>[2x]SMANLRKVLISDSLDPCCRKILQDGGLQVVEKQNLSKEELIAELQDCEGLIVRSATKVTADVINAAEKLQVVGRAGTGVDNVDLEAATRKGILVMNTPNGNSLSAAELTCGMIMCLARQIPQATASMKDGKWERKKFMGTELNGKTLGILGLGRIGREVATRMQSFGMKTIGYDPIISPEVSASFGVQQLPLEEIWP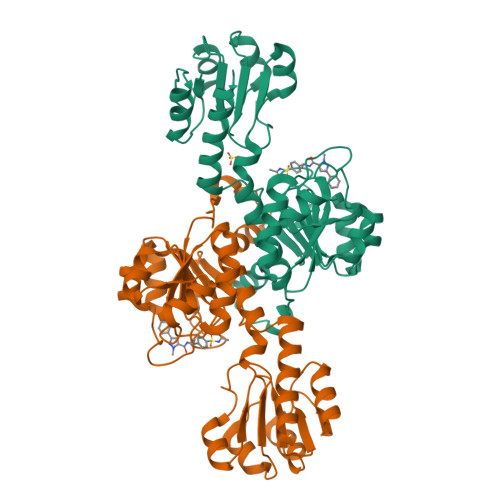LCDFITVHTPLLPSTTGLLNDNTFAQCKKGVRVVNCARGGIVDEGALLRALQSGQCAGAALDVFTEEPPRDRALVDHENVISCPHLGASTKEAQSRCGEEIAVQFVDMVKGKSLTGV> EQRRLYDQAKAALAKGNSAPYMASRSALRDYPLEPYLAYDELTHRLKSASNEEVERFLTEHGDLPQIGWLKLRWLRLLADRGDWKTFVNYYDPKLNFTELDCLYGQYQLGHGQKAEGYATSERLWLVGKSQPAACDTLFGLWQGEGQLTEEKVWKRLKLAAEARNYSLASHLAQRLPTLGNQGALMVSVAQNPAQLSQTGRFSQRDHATADVVGLGLRRLARQDPEKALSLLDYYSSALPFSSDEKVAIAREIGLSLAKRFDPRALPLMTQYDPGLRDNTVTEWRTRLLLRLGRWDEAYALTRKLPQDLAATSRWRYWQARSLQLAQPNSKEPIALYQKLAGERDFYGFLAADRLSVPYKLGNRPAHIDPRVLQRVRNAASTRRAMEFFNRGEVINARREWYHAARLFDRDELIAQARLAYDMQWYFPAIRSISQAQYWDDLDIRFPMAHRATLVREAKNRGLHSSWIFAITRQQSAFMSDARSGVGATGLMQLMPGTAKETSRKFGIPLASTQQLIVPDVNIRLGAAYLSQVHSQFNGNRVLAS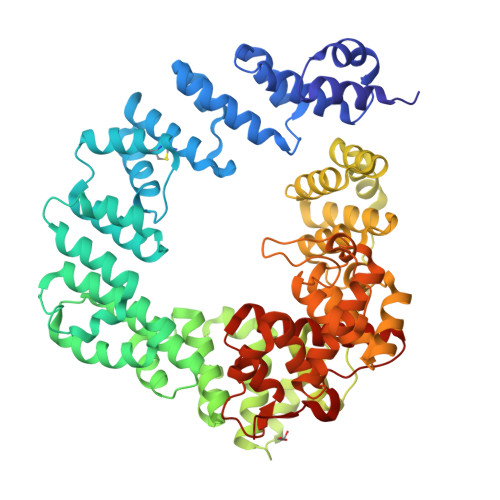AAYNAGPGRVRQWLKDTRHLAFDVWIETIPFDETRQYVQNVLSYAVIYGQKLNAPQPIVDWHERYFDDF> ASLNGTLMQYFEWYMPNDGQHWKRLQNDSAYLAEHGITAVWIPPAYKGTSQDDVGYGAYDLYDLGEFHQKGTVRTKYGTKGELQSAINSLHSRDINVYGDVVINHKGGADATEYVTAVEVDPADRNRVTSGEQRIKAWTHFQFPGRGSTYSDFKWYWYHFDGTDWDESRKLNRIYKFQGKAWDWEVSNENGNYDYLMYADIDYDHPDVTAEIKRWGTWYANELQLDGFRLDAVKHIKFSFLRDWVNHVREKTGKEMFTVAEYWQNDLGALENYLNKTNFNHSVFDVPLHYQFHAASTQGGGYDMRKLLNGTVVSKHPVKAVTFVDNHDTQ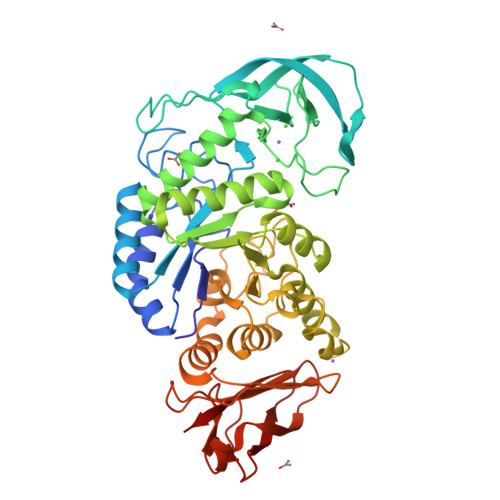PGQSLESTVQTWFKPLAYAFILTREAGYPQIFYGDMYGTKGASQREIPALKHKIEPILKARKQYAYGAQHDYFDHHNIVGWTREGDSSVANSGLAALITDGPGGTKRMYVGRQNAGETWHDITGNRSDSVVINAEGWGEFHVNGGSVSIYVQR>GSSHHHHHHSQDLEVLFQGPHMAGFKRGYDGKIAGLYDLDKTLGRGHFAVVKLARHVFTGEKVAVKVIDKTKLDTLATGHLFQEVRCMKLVQHPNIVRLYEVIDTQTKLYLILELGDGGDMFDYIMKHEEGLNEDLAKKYFAQIVHAISYCHKLHVVHRDLKPENVVFFEKQGLVKLTDFGFSNKFQPGKKLTTSCGSLAYSAPEILLGDEYDAPAVDIWSLGVILFMLVCGQPPFQEANDSETLTMIMDCKYTVPSHVSKECKDLITRMLQRDPKRRASLEEIENHPWLQGVDPSPATKYNIPLVSYKNLSEEEHNSIIQRMVLGDIADRDAIVEALETN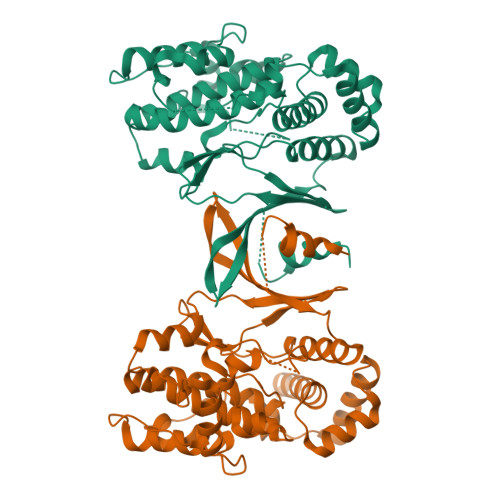RYNHITATYFLLAERILREKQEKEIQTRSASPSNIK[2x]> GAMSSIFINREYLLPDYIPDELPHREDQIRKIASILAPLYREEKPNNIFIYGLTGTGKTAVVKFVLSKLHKKFLGKFKHVYINTRQIDTPYRVL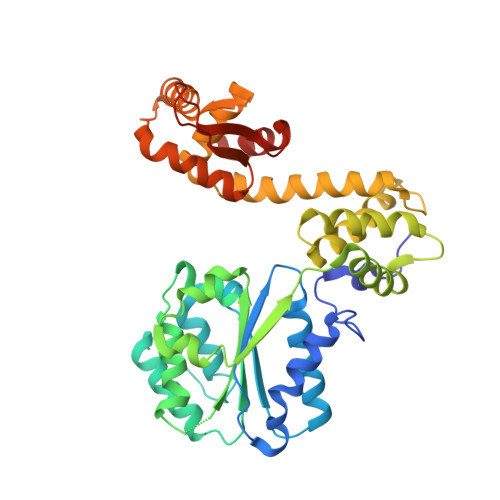ADLLESLDVKVPFTGLSIAELYRRLVKAVRDYGSQVVIVLDEIDAFVKKYNDDILYKLSRINSEVNKSKISFIGITNDVKFVDLLDPRVKSSLSEEEIIFPPYNAEELEDILTKRAQMAFKPGVLPDNVIKLCAALAAREHGDARRALDLLRVSGEIAERMKDTKVKEEYVYMAKEEIERDRVRDIILTLPFHSKLVLMAVVSISSEENVVSTTGAVYETYLNICKKLGVEAVTQRRVSDIINELDMVGILTAKVVNRGRYGKTKEIGLAVDKNIIVRSLIESDSRFADLWS2-[4-({5-amino-3-[(4-sulfamoylphenyl)amino]-1H-1,2,4-triazole-1-carbonyl}amino)phenyl]-1,3-oxazole-4-carboxylic acid | C19 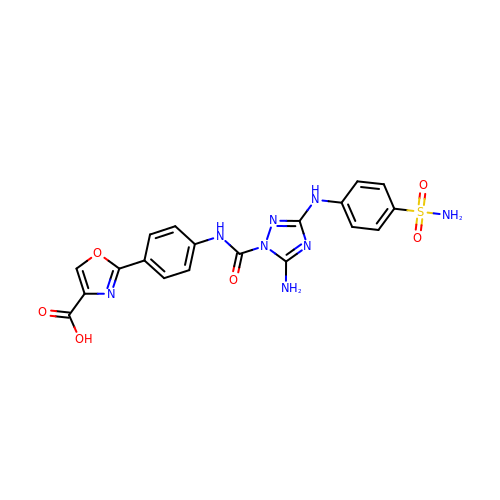H16 N8 O6 S | SCZCTYREODBPFV-UHFFFAOYSA-N> IKELKMSKDEIKREYKEMEGSPEIKSKRRQFHQEI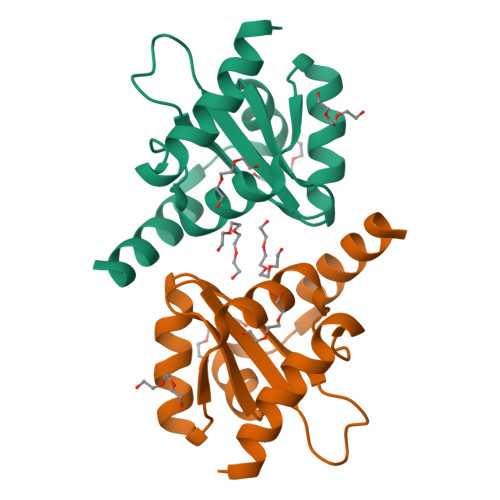QSRNMRENVKRSSVVVAAPTHIAIGILYKRGETPLPLVTFKYTDAQVQTVRKIAEEEGVPILQRIPLARALYWDALVDHYIPAEQIEATAEVLRWLERQNIEKQHSEML> IVGEALEYVNIGLS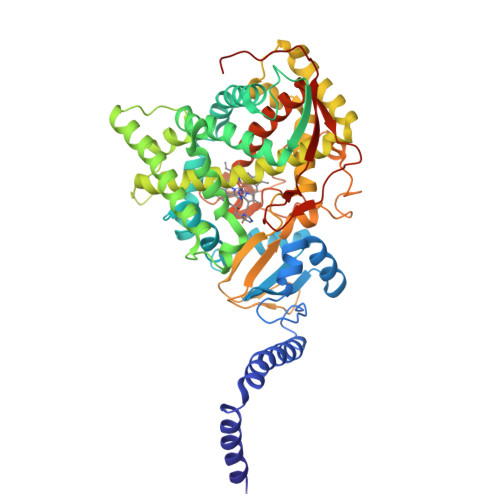HFLALPLAQRISLIIIIPFIYNIVWQLLYSLRKDRPPLVFYWIPWVGSAVVYGMKPYEFFEECQKKYGDIFSFVLLGRVMTVYLGPKGHEFVFNAKLADVSAEAAYAHLTTPVFGKGVIYDCPNSRLMEQKKFVKGALTKEAFKSYVPLIAEEVYKYFRDSKNFRLNERTTGTIDVMVTQPEMTIFTASRSLLGKEMRAKLDTDFAYLYSDLDKGFTPINFVFPNLPLEHYRKRDHAQKAISGTYMSLIKERRKNNDIQDRDLIDSLMKNSTYKDGVKMTDQEIANLLIGVLMGGQHTSAATSAWILLHLAERPDVQQELYEEQMRVLDGGKKELTYDLLQEMPLLNQTIKETLRMHHPLHSLFRKVMKDMHVPNTSYVIPAGYHVLVSPGYTHLRDEYFPNAHQFNIHRWNNDSASSYSVGEEVDYGFGAISKGVSSPYLPFGGGRHRCIGEHFAYCQLGVLMSIFIRTLKWHYPEGKTVPPPDFTSMVTLPTGPAKIIWEKRNPEQKIGGRH>SNAMGQVRGAAGVTDGNEVAKAQQATPGGAAPTIFSRILDKSLPADILYEDQQCLV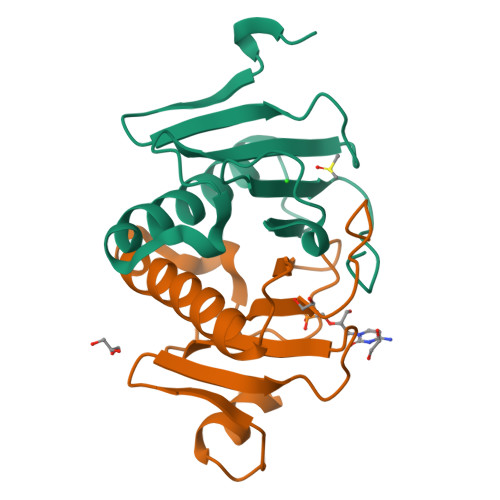FRDVAPQAPVHFLVIPKKPIPRISQAEEEDQQLLGHLLLVAKQTAKAEGLGDGYRLVINDGKLGAQSVYHLHIHVLGGRQLQWPPG[2x]> MEEVTFRIAPEEKVKKKPSFLKPWFGLKYLFKKPVTIKIPYEFIEPAPRYRGFHTLDWKKCIGCNMCGQICPARAIEMTWIEGEKRPHPKIDYGRCTFCQFCVDVCPTGALGFIETYMLTTTWREEELLLYDWVPIEPEKFKEIQEKFKDYKF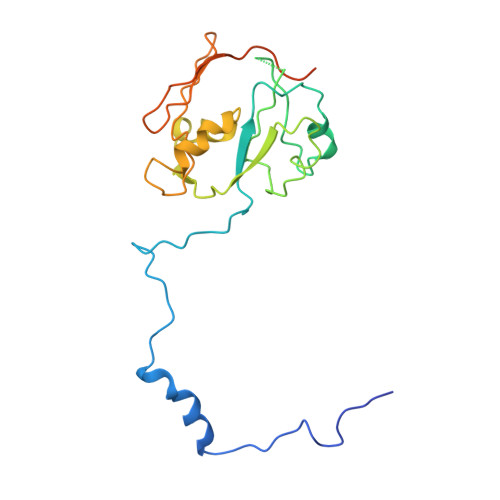PVEKIEFNKETKEVTYYLRDGTTFKFKILGYGLKPPVKPQPTTKQQEEEKKESGQ> MKHFTAA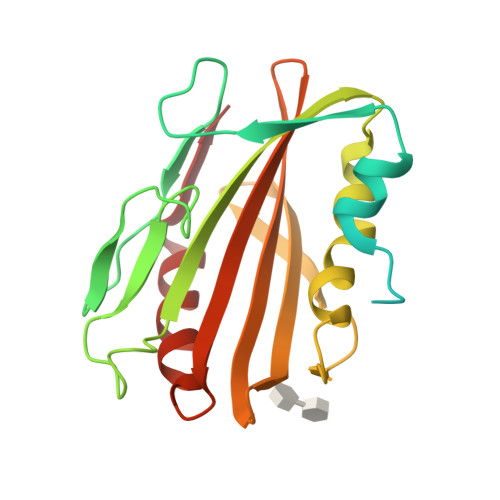VATVALSLALAGCSFNIKTDSAPTTSPTTTSPTTSTTTTSATTSAQAAGPNYTIADYIRDNHIQETPVHHGDPGSPTIDLPVPDDWRLLPESSRAPYGGIVYTQPADPNDPPTIVAILSKLTGDIDPAKVLQFAPGELKNLPGFQGSGDGSAATLGGFSAWQLGGSYSKNGKLRTVAQKTVVIPSQGAVFVLQLNADALDDETMTLMDAANVIDEQTTITP> GDEPSDLEELEKFAKTFKQRRIKLGFTQGDVGLAMGKLYGNDFSQTTISRFEALNLSFKNMCKLKPLLEKWLNDAESSPSDPSVSTPSSYPSLSEVFGRKRKKRTSIETNIRLTLEKRFQDNPKPSSEEIS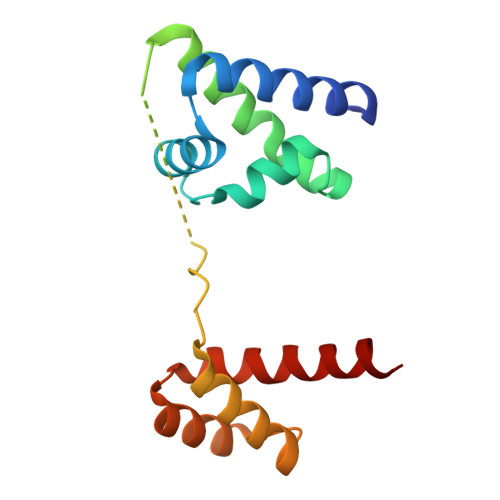MIAEQLSMEKEVVRVWFCNRRQKEKRINC> MDSTKEKCDSYKDDLLLRMGLNDNKAGMEGLDKEKINKIIMEATKGSRFYGNELKKEKQVNQRIENMMQQKAQITSQQLRKAQLQVDRFAMELEQSRNLSNTIVHIDMDAFYAAVEMRDNPELKDKPIAVGSMSMLSTSNYHARRFGVRAAMPGFIAKRLCPQLIIVPPNFDKYRAVSKEVKEILADYDPNFMAMSLDEAYLNITKHLEERQNWPEDKRRYFIKMGSSVENDNPGKEVNKLSEHERSISPLLFEESPSDVQPPGDPFQVNFEEQNNPQILQNSVVFGTSAQEVVKEIRFRIEQKTTLTASAGIAPNTMLAKVCSDKNKPNGQYQILPNRQAVMDFIKDLPIRKVSGIGKVTEKMLKALGIITCTELYQQRALLSLLFSETSWHYFLHISLGLGSTHLTRDGERKSMSVERTFSEINKAEEQYSLCQELCSELAQDLQKERLKGRTVTIKLKNVNFEVKTRASTVSSVVSTAEEIFAIAKELLKTEIDADFPHPLRLRLMGVRISSFPNEEDRKHQQRSIIGFLQAGNQALSATECTLEKTDKDKFVKPLEMSHKKSFFDKKRSERKWSHQDTFKCEAVNKQSFQTSQPFQVLKKKMNENLEISENSDDCQILTCPVCFRAQGCISLEALNKHVDECLDGPSISENFKMFSCSHVSATKVNKKENVPASSLCEKQDYEAHPKIKEISSVDCIALVDTIDNSSKAESIDALSNKHSKEECSSLPSKSFNIEHCHQNSSSTVSLENEDVGSFRQEYRQPYLCEVKTGQALVCPVCNVEQKTSDLTLFNVHVDVCLNKSFIQELRKDKFNPVNQPKESSRSTGSSSGVQKAVTRTKRPGLMTKYSTSKKIKPNNPKHTLDIFFK;>GPHMFEARLVQGSILKKVLEALKDLINEACWDISSSGVNLQSMDSSHVSLVQLTLRSEGFDTYRCDRNLAMGVNLTSMSKILKCAGNEDIITLRAEDNADTLALVFEAPNQEKVSDYEMKLMDLDVEQLGIPEQEYSCVVKMPSGEFARICRDLSHIGDAVVISCAKDGVKFSASGELGNGNIKLSQTSNVDKEEEAVTIEMNEPVQLTFALRYLNFFTKATPLSSTVTLSMSADVPLVVEYKIADMGHLKYYLAPKIEDEEGS[3x]

Y-family DNA polymerase κ (Pol κ) can replicate damaged DNA templates to rescue stalled replication forks. Access of Pol κ to DNA damage sites is facilitated by its interaction with the processivity clamp PCNA and is regulated by PCNA mono-ubiquitylation. In this work, we present cryo-EM reconstructions of full-length human Pol κ bound to a primer/template (P/T) DNA substrate, an incoming nucleotide, and wild-type PCNA (wt-PCNA) or PCNA mono-ubiquitylated at K164 (Ub-PCNA), at resolutions between ~3.4 and ~6.4 Å. The structures of the complexes with either wt-PCNA or Ub-PCNA are very similar and show the Pol κ core docked to one PCNA protomer through the internal PIP-box adjacent to the PAD.

We reconstituted the Pol κ−DNA−wt-PCNA complex by mixing purified recombinant Pol κ, PCNA, a (25/38) P/T DNA substrate containing a dideoxy chain terminator in the primer strand, and dTTP as the incoming nucleotide. The complex was separated by micro-size exclusion chromatography, vitrified and imaged by cryo-EM. We obtained a reconstruction of the complex at a global resolution of 3.4 Å (Fig. 1c−e). The structure has approximate dimensions of 127.7 × 88.0 × 89.1 Å, and displays the catalytic core of Pol κ sitting on top of the front face of PCNA in a remarkably angled orientation, with the axis of DNA in the catalytic cleft tilted by ~47° relative to the normal of the PCNA ring plane. The duplex DNA emerging from the catalytic core threads through the PCNA ring hole and bends by ~30° to avoid clashing with the ring inner rim. The long region C-terminal to the PAD (residues 535−870) is invisible in the map, suggesting it is flexible, in agreement with the disorder prediction. Specifically, residues 518−525 fold into a two-turn α-helix (“Inverting helix”), which reverses the chain direction and inserts the PIP-box (526QRSIIGFL) between the loop connecting helix αQ and β11 of the PAD, the hydrophobic cleft on the front face of PCNA, and the PCNA C-terminus. The PIP-box acquires the canonical 3.10 helix conformation and docks to the PCNA groove via a three-fork plug made of side chains of Ile529, Phe532 and Leu533, while Gln526 binds in the so-called “Q-pocket”. Thus, the folding and concomitant insertion of the PAD C-terminus between the PAD and PCNA creates a composite interface burying a total of 733 Å2, and bends Pol κ core over the bound PCNA protomer, causing the bending of DNA threading the PCNA pore. In the active site of Pol κ, Watson−Crick base pairing is observed between the incoming dTTP and the opposing A in the template strand. The triphosphate of dTTP inserts between the palm and fingers domain and its position is locked by hydrogen bonding with Tyr111, Arg144 and Lys328, three conserved residues among Y-family polymerases.>[2x]MSLAMQDFRP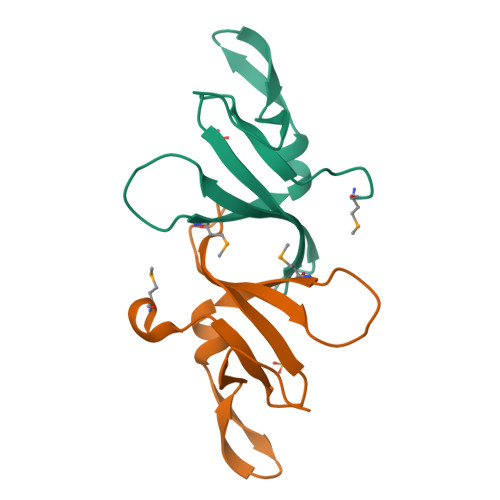GVYRHYKGDHYLALGLARADETDEVVVVYTRLYARAGLPMSTRLLRIWNETVDTGAGPQPRFAYVGHVTPEQGEGHHHHHH>GAHMNDIKQLLWNGELNVLVSIDPSFLMKGSPREIAVLRIRVPRETYLVNYMPLIWNKIKSFLSFDPLTDSEKYFWFEHNKTPIPWNYPVGVLFDCLAGKSATFTTSFENQVKDVLTFLRIHLVMGDSLPPTIIPIASSKTQAEKFWFHQWKQVCFILNGSSKAIMSLSVNEARKFWGSVITRNFQDFIEISNKISSSRPRHIPLIIQTSRTSGTFRISQP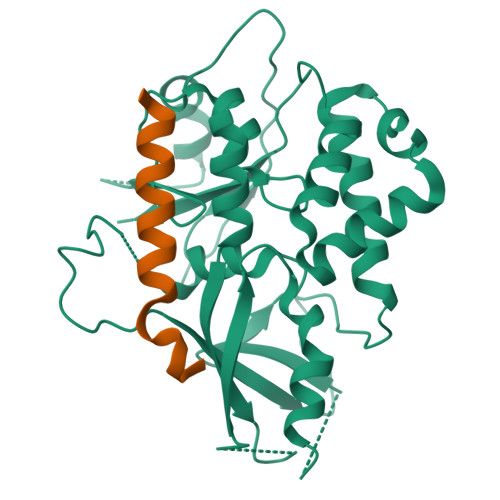TISMTGVNPTLKDIEGDILDVKEGINGNDVMVICQGIEIPWHMLLYDLYSKLRSFDGFLYITLVPIKGGDKASSEL[4x];>MGNFIITERKKAKEERSNPQTDSMDDLLIRRLTDRNDKEAHLNELF[4x]> MPIIIDKDLPARKVLQEENIFVMTKERAETQDIRALKIAILNLMPTKQETEAQLLRLIGNTPLQLDVHLLHMESHLSRNVAQEHLTSFYKTFRDIENEKFDGLIITGAPVETLSFEEVDYWEELKRIMEYSKTNVTSTLHICWGAQAGLY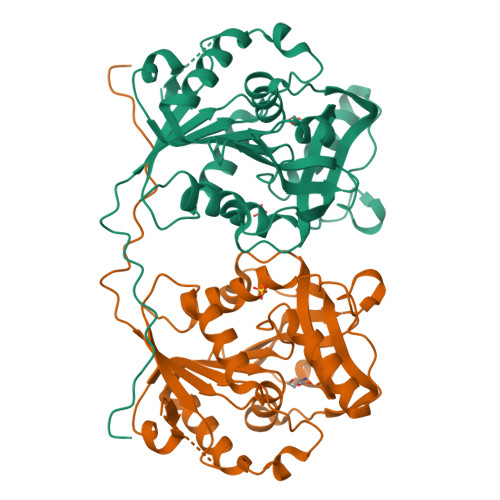HHYGVQKYPLKEKMFGVFEHEVREQHVKLLQGFDELFFAVHSRHTEVRESDIREVKELTLLANSEEAGVHLVIGQEGRQVFALGHSEYSCDTLKQEYERDRDKGLNIDVPKNYFKHDNPNEKPLVRWRSHGNLLFSNWLNYYVYQETPYVL> MQSTVHIVGDNTGWSVPSSPNFYSQWAAGKTFRVGDSLQFNFPANAHNVHEMET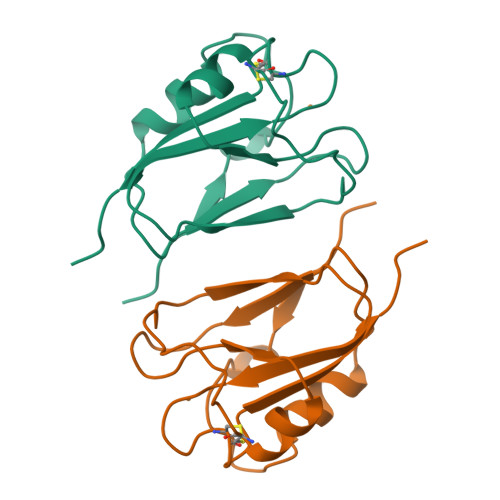KQSFDACNFVNSDNDVERTSPVIERLDELGMHYFVCTVGTHCSNGQKLSINVVAANATVSMPPPSSSPPSSVMPPPVMPPPSPS>[2x]SDKIIHLTDDSFDTDVLKADGAILVD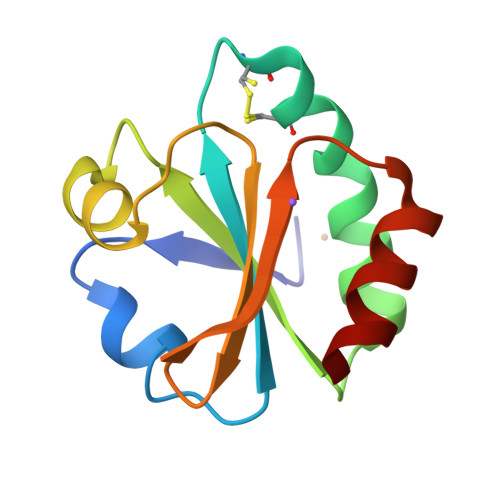FWAEWCGACKMIAAILDEIADEYQGKLTVAKLNIDQNAGTAAKYGIRGIPTLLLFKNGEVAATKVGALSKGQLKEFLDANLA>MDLADRFAELERRYDARLGVYVPATGTTAAIEYRADERFAFCSTFKAPLVAAVLHQNPLTHLDKLITYTSDDIRSISPVAQQHVQTGMTIGQLCDAAIRYSDGTAANLLLADLGGPGGGTAAFTGYLRSLGDTVSRLDAEEPELNRDPPGDERDTTTPHAIALVLQQL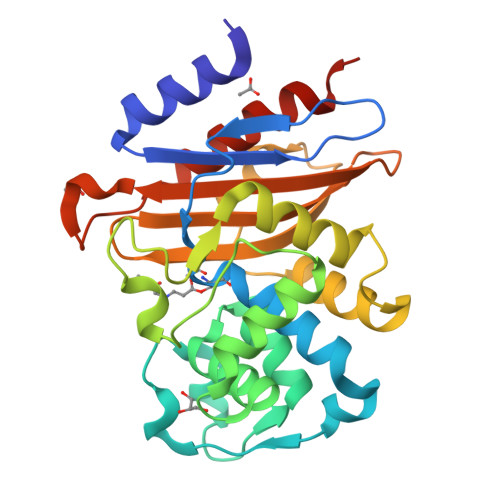VLGNALPPDKRALLTDWMARNTTGAKRIRAGFPADWKVIDKTGTGDYGRANDIAVVWSPTGVPYVVAVMSDRAGGGYDAEPREALLAEAATCVAGVLALEHHHHHH[2x]(3R)-3-[[(3S)-3-ethylpiperidin-1-yl]methyl]-6,8-bis(oxidanyl)-3,4-dihydroisochromen-1-one 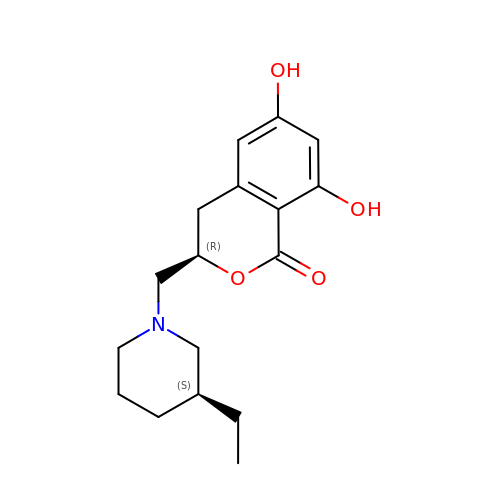| C17 H23 N O4 | PVQQYHLNENIZDV-SMDDNHRTSA-N>MFTGSIVAIVTPMDEKGNVCRASLKKLIDYHVASGTSAIVSVGTTGESATLNHDEHADVVMMTLDLADGRIPVIAGTGANATAEAISLTQRFNDSGIVGCLTVTPYYNRPSQEGLYQHFKAIAEHTDLPQILYNVPSHTGCDLLPETVGRLAKVKNIIGIKEATGNLTRVNQIKELVSDDFVLLSGDDASALDFMQLGGHGVISVTANVAARDMAQMCKLAAEGHFAEARVINQRLMPLHNKLFVEPNPIPVKWACKELGLVATDTLRLPMTPITDSGRETVRAALKHAGLL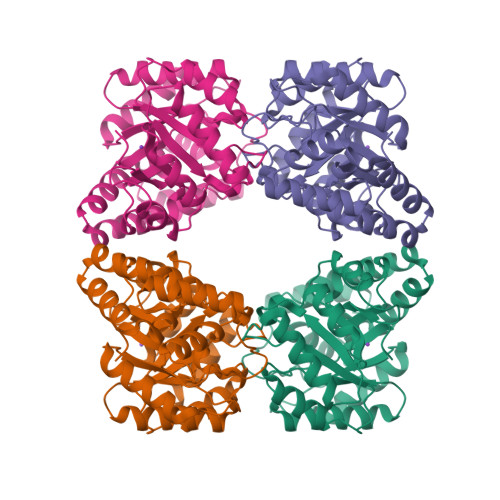[2x]> GAMGSILDPEVLKVAEYVYQERLSKPY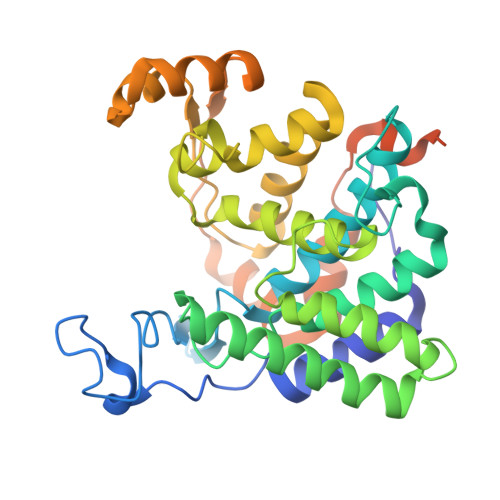TEVGPEWEYNHKTPYATRATGTGHNLQRFITIDDQRLHRPIHGLAHTMRTLFYSQLMYEAAKRQPHPHRCADGRTIADLSVQDLKKLNIAQLFFVAGRESEASYGDAYHRYHLYGAKQFEAYARKHLTHLFSEKEIVLYSRCIEDRIGDRFDETAEGYLIHLSHMIDLMRCKSPVEVFIGHSRGVSGIVPTLIQLFGREDGLDIMHYARSLFAATGEAVPYISSSEWPHLGIESDRVERALKIVGSLEVEGQEADAKKTAQAGFSVDGCYGALVKIDTPDWYHQVKEKEDYDVDEVIALPPQITIREEPPKTNESFLLSL> MTIDEIIEAIEKLT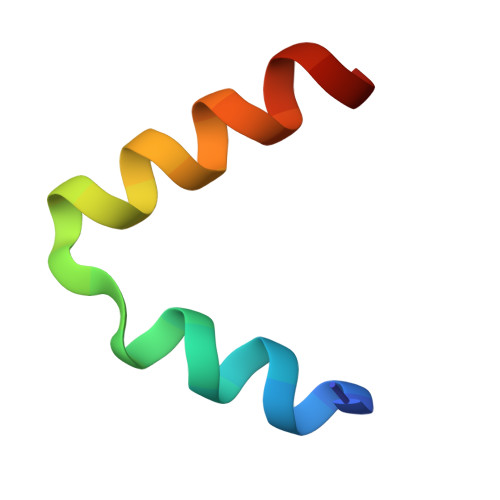VSELAELVKKLEDKFG> MVLEVYYTSLRCRCVQESSVFIPRRFIDRIQILPRGNGCPRKEIIVWKKNKSIVCVDPQAEWIQRMMEVLRKRSSSTLPVPVFKRKIP

CXCL13 is the cognate chemokine agonist of CXCR5, a class A G-protein-coupled receptor (GPCR) that is essential for proper humoral immune responses. CXCL13 is an agonist of CXCR5, activating the receptor, resulting in downstream calcium signaling and ultimately the chemotactic response for which chemokines are named. As elucidated from structural data on many chemokines, this conserved tertiary structure consists of a disordered N-terminal region (6–10 amino acids, referred to here as the chemokine N-terminus), followed by a long loop known as the ‘N-loop’ ending in a short 310-helix, a three-stranded β-sheet and a C-terminal α-helix. Furthermore, we were able to utilize two of these mutants to solve the first uncomplexed crystal structures of human CXCL13. These structures allowed us to observe that the core domain of CXCL13 (i.e. everything except its N- and C-termini) is fairly rigid, whereas its N-terminus exhibits striking flexibility as well as a propensity to form both intramolecular and intermolecular β-strand interactions.

Upon administering both WT and Met CXCL13 to these cells in a dose-dependent manner, we observed that both functioned as agonists, albeit with differing potencies and efficacies. In particular, we found that WT CXCL13 had an observed half-maximal effective concentration (EC50) value of 2.49 nM, whereas Met CXCL13 had an EC50 of 26.3 nM. In terms of efficacy, we defined the maximum activity elicited by WT CXCL13 acting on CXCR5 at the highest concentration tested (1 µM) to be 100% (defining it as a full agonist) and our negative control of buffer alone to equate to 0% activity; our receptor-independent positive control, 2 µM ionomycin, produced a response of ∼119.6% relative to WT CXCL13 (data not shown). Using these parameters, we observed that Met CXCL13 had a maximum efficacy of 86.8% when administered at 1 µM, classifying it as a partial agonist of CXCR5. We were able to solve the crystal structure of Met CXCL13 to 1.88 Å resolution. We utilized the structure of CXCL10 [chemokine (C-X-C) motif ligand 10] to perform molecular replacement and generate an initial model that was then iteratively refined to generate the final structure. Further inspection of Met CXCL13 indicated that there is one monomer per asymmetric unit that forms a crystallographic dimer with a symmetry mate. We next observed the specific interactions that allow the formation of the β0 strand in the Met CXCL13 structure. One set of interactions are the typical hydrogen bonds formed between the β0 and β1 strands to create the parallel β-strand interaction and the four-stranded β-sheet. We also observed that the initiating methionine itself (Met0) was responsible for helping to stabilize this unique feature with both intermolecular and intramolecular interactions.>QDRLDAPPPPAPPLLRWAGPVGVSWGLRAAAPGGPVPRAGRWRRGAPAEDQDCGRLPDFIAKLTNNTHQHVFDDLSGSVSLSWVGDS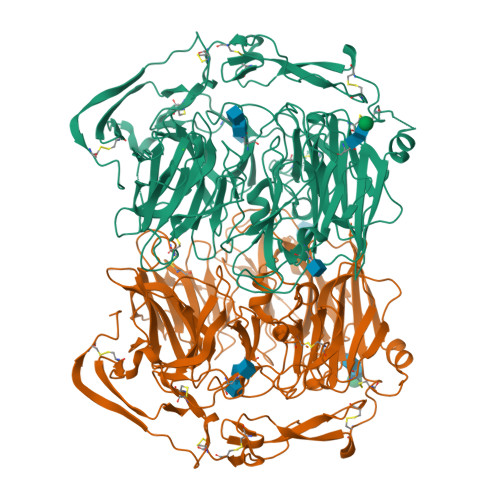TGVILVLTTFQVPLVIVSFGQSKLYRSEDYGKNFKDITNLINNTFIRTEFGMAIGPENSGKVILTAEVSGGSRGGRVFRSSDFAKNFVQTDLPFHPLTQMMYSPQNSDYLLALSTENGLWVSKNFGEKWEEIHKAVCLAKWGPNNIIFFTTHVNGSCKADLGALELWRTSDLGKTFKTIGVKIYSFGLGGRFLFASVMADKDTTRRIHVSTDQGDTWSMAQLPSVGQEQFYSILAANEDMVFMHVDEPGDTGFGTIFTSDDRGIVYSKSLDRHLYTTTGGETDFTNVTSLRGVYITSTLSEDNSIQSMITFDQGGRWEHLRKPENSKCDATAKNKNECSLHIHASYSISQKLNVPMAPLSEPNAVGIVIAHGSVGDAISVMVPDVYISDDGGYSWAKMLEGPHYYTILDSGGIIVAIEHSNRPINVIKFSTDEGQCWQSYVFTQEPIYFTGLASEPGARSMNISIWGFTESFITRQWVSYTVDFKDILERNCEEDDYTTWLAHSTDPGDYKDGCILGYKEQFLRLRKSSVCQNGRDYVVAKQPSVCPCSLEDFLCDFGYFRPENASECVEQPELKGHELEFCLYGKEEHLTTNGYRKIPGDKCQGGMNPAREVKDLKKKCTSNFLNPTKQNSKSNAAAHHHHHH[2x]In this work, we exhaustively probe the ability of all 36 immobile HJ sequences to form DNA crystals in two different designed systems. Three separate self-assembling DNA crystal systems are described in this report: the “4 × 5” and “4 × 6” designs (collectively referred to as the 4 × N systems), and a third construct with a “scrambled” sequence variant of the 4 × 6 lattices. Self-assembly was mediated by three constituent oligonucleotides: (S1) containing four sequence repeats of either 5 or 6 bases; (S2) composed of 21 bases containing complementary regions to both (S1); and (S3) which forms the second junction crossover. The HJ serves as the fundamental component at the core of each unit, and the ultimate assembly of the full lattice is facilitated by the complementary 2-base sticky ends that tail each duplex.

The 4 × 5 system robustly crystallized with 75% of the junctions, and we obtained crystals in all but 9 of 36 sequences. Of the resulting structures, 18 exhibited P32 symmetry with average cell dimensions a = b = 68.85 Å c = 60.09 Å, with only nine retaining the original P3221 symmetry with average cell edges a = b = 68.17 Å c = 60.60 Å. Although the cell parameters between the two symmetries were virtually indistinguishable, the differences between the periodicity of the lattices is dramatic, with vastly different cavity sizes. While the highest resolution achieved for the J1 system was 3.1 Å, in roughly half of the crystals measured the resolutions were 3.05 Å or better, and as high as 2.9 Å (J6) and 2.75 Å (J19), for the P32 and P3221 symmetries, respectively.

> GAGCAGACGAG;> ACTCCACTCA;> CTAGT;> TCTGAGTGGCGTCTGC> SLRPPLPPATPQEVQFVQHMLQHHAQALDLAAPMLERSQQRTVRSLALDIQLSQREQMRQMEAMLGRWGQPPGEPISPEHARMMGMASEAEV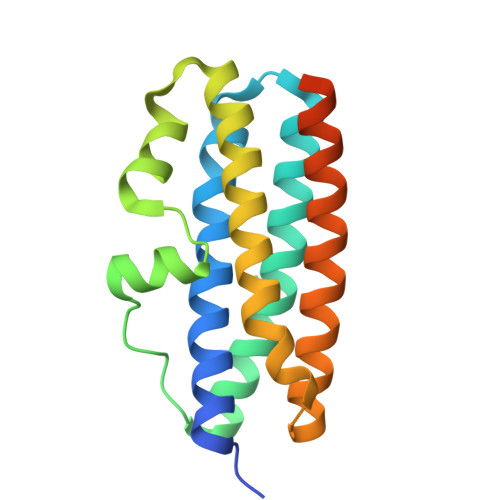AGLSTLPVEQAERQFLRLMIRHHQGAVAMTLPMLDAAARPEVERLARQIVVTQRGEIRTMEGVLGRLDGEVPAAPMRPVEHGHGH>[2x]VIDLNASAQAMSDLDEGAINEVVDKVMAKADADAAQELIKAFQQGMTKV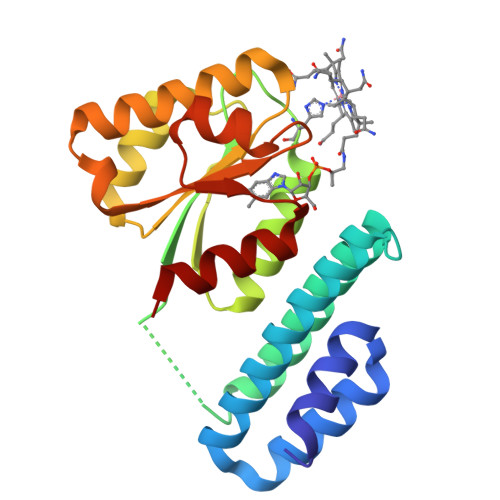GERFDSGEYFIGDLIFAGEILQAAMDKLKPALSGDALEKRAKIVLATVEGDLHDIGKNIFRTMAEASGFEVFDLGIDVPVKIIVDKVKEVNPEIVGLSGVLTLALDSMRETVDALKAEGLRNDLKVIIGGVPVNENVCQRVGADDFSTNAADGVKICQRWVG>[2x]GCUTAATUCG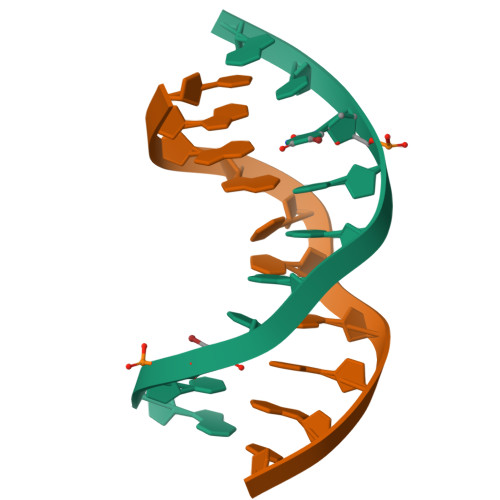;>[2x]CGAATTAAGC>[6x]MGHHHHHHSGENLYFQGASMRTLLIRYILWRNDGDPSYYNDDFKKLILFDELVDDDDVCTLIKNMRM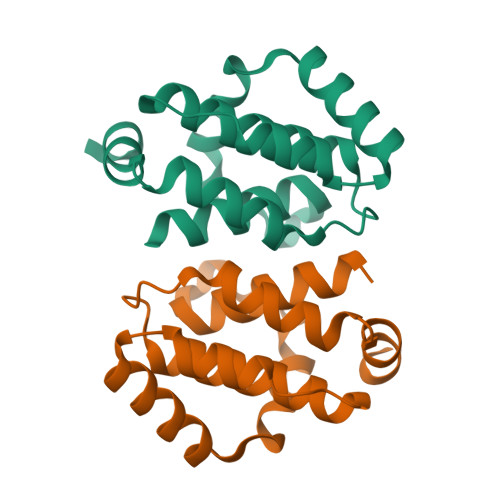TLSDGPLLDRLNQPVNNVEDVKRMIAISAKVARDIGRRSEIRWEDSFTILFRMIEKYFDDLMTDLYGEK>[2x]TATYSGNPFVGVTPWANAYYASEVSSLAIPSLTGAMATAAAAVAKVPSFMWLDTLDKTPLMEQTLADIRTA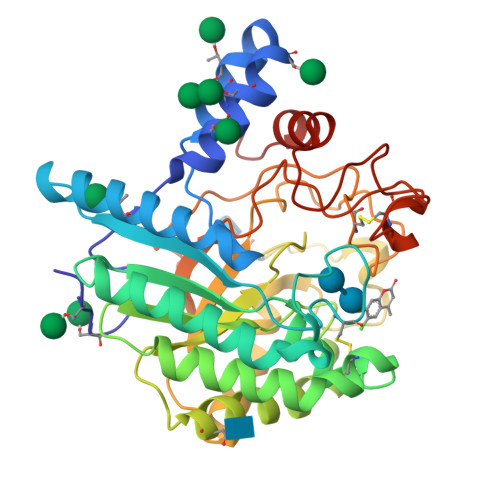NKNGGNYAGQFVVYDLPDRDCAALASNGEYSIADGGVAKYKNYIDTIRQIVVEYSDIRTLLVIEPASLANLVTNLGTPKCANAQSAYLECINYAVTQLNLPNVAMYLDAGHAGWLGWPANQDPAAQLFANVYKNASSPRALRGLATNVANYNGWNITSPPSYTQGNAVYNEKLYIHAIGPLLANHGWSNAFFITDQGRSGKQPTGQQQWGDWCNVIGTGFGIRPSANTGDSLLDSFVWVKPGGECDGTSDSSAPRFDSHCALPDALQPAPQAGAWFQAYFVQLLTNANPSFL> PLGSATITQDTPINQIFTDTALAEKMKTVLGKTNVTDTVSQTDLDQVTTLQADRLGIKSIDGVEYLNNLTQINFSNNQLTDITPLKNLTKLVDILMNNNQIADITPLANLTNLTGLTLFNNQITDIDPLKNLTNLNRLELSSNTISDISALSGLTSLQQLSFGNQVTDLKPLANLTTLERLDISSNKVSDISVLAKLTNLESLIATNNQISDITPLGILTNLDELSLNGNQLKDIGTLASLTNLTDLDLANNQISNLAPLSGLTKLTELKLGANQISNISPLAGLTALTNLELNENQLEDISPISNLKNLTYLTLYFNNISDISPVSSLTKLQRLFFANNKVSDVSSLANLTNINWLSAGHNQISDLTPLANLTRITQLGLNDQAWTNAPVNYKANVSIPNTVKNVTGALIAPATISDGGSYTEPDITWNLPSYTNEVSYTFSQPVTIGKGTTTFSGTVTQPLKGG;> GPLGSWVIPPISCPENEKGPFPKNLVQIKSNKDKEGKVFYSITGQGADTPPVGVFIIERETG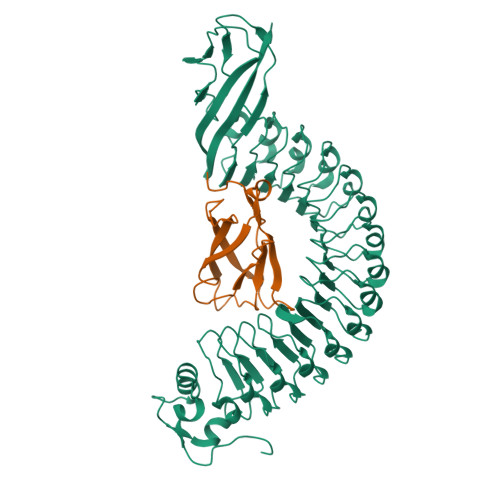WLKVTEPLDRERIATYTLFSHAVSSNGNAVEDPMEILITVTDQ> MKFLKNVLEEGSKLEEFNELELSPEDKELLEYLQQTKAKITVVGCGGAGNNTITRLKMEGIEGAKTVAINTDAQQLIRTKADKKILIGKKLTRGLGAGGNPKIGEEAAKESAEEIKAAIQDSDMVFITCGLGGGTGTGSAPVVAEISKKIGALTVAVVTLPFVMEGKVRMKNAMEGLERLKQHTDTLVVIPNEKLFEIVPNMPLKLAFKVADEVLINAVKGLVELITKDGLINVDFADVKAVMNNGGLAMIGIGESDSEKRAKEAVSMALNSPLLDVDIDGATGALIHVMGPEDLTLEEAREVVATVSSRLDPNATIIWGATIDENLENTVRVLLVITGVQSRIEFTDTGLKRKKLELTGI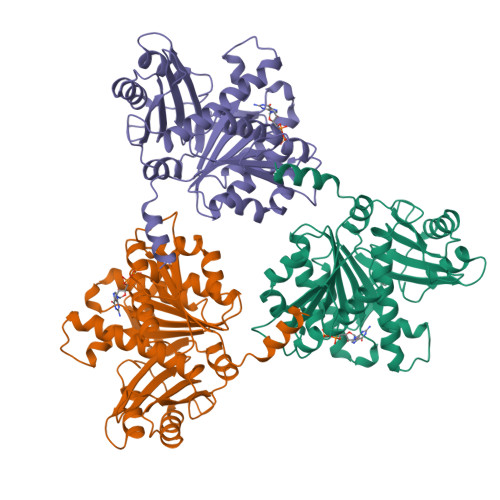PKIGSHHHHHH> YFW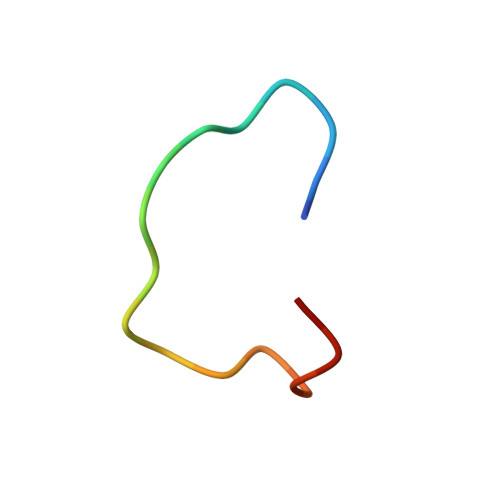GNLHWYYEQFDSTCX> RAVDLVDDSNDVDNSIEAEEEKPRNRAFEADWLKFTKTPPTKLQQADGATIEIVCEMMGSQVPSIQWVVGHLPRSELDDLDSNQVAEEAPSAIVRVRSSHIIDHVLSEARTYTCVGRTGSKTIYASTVVHPPRSSRLTPEKTYPGAQKPRIIYTEKTHLDLMGSNIQLPCRVHARPRAEITWLNNENKEIVQGHRHRVLA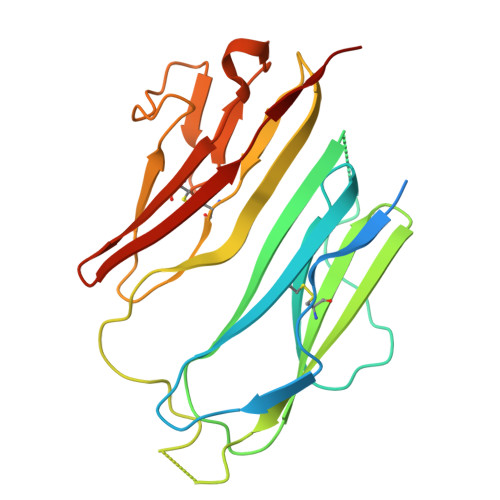NGDLLISEIKWEDMGNYKCIARNVVGKDTADTFVYPVLNEED> MAQKPVADALTLELEPVVEANMTRHLDTEDIWFAHDYVPFDQGENFAFLGGRDWDPSQSTLPRTITDACEILLILKDNLAGHHRELVEHFILEDWWGRWLGRWTAEEHLHAIALREYLVVTREVDPVANEDVRVQHVMKGYRAEKYTQVETLVYMAFYERCGAVFCRNLAAQIEEPILAGLIDRIARDEVRHEEFFANLVTHCL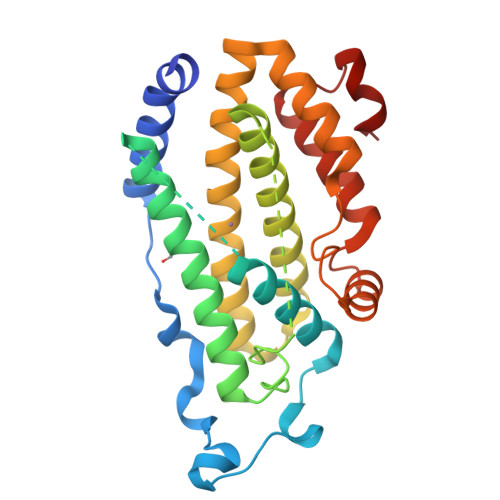DYTRDETIAAIAARAADLDVLGADIEAYRDKLQNVADAGIFGKPQLRQLISDRITAWGLAGEPSLKQFVTG>MALLTPIPSPMVNLTQVIDPTEQLAYFPKITFERLKNYDTSSNYAKGKLTRNYMILLPWQHVNRYNFVFSSTGCKVSLKTCIGKLMKDLNPKVLYFIGEGAGNWMARTACEYPDIKFVYRSLKDDLDHHYPLEYQRVIGELSRIIDSGEGLSMETTDATQKTHWDLIHRVSKDALLITLCDAEFKDRDDFFKMVILWRKHVLSCRICTTYGTDLYLFAKYHAKDCNVKLPFFVRSVATFIMQGSKLSGSECYILLTLGHHNNLPCHGEIQNSKMKIAVCNDFYAAKKLDNKSIEANCKSLLSGLRIPINKKELNRQRRLLTLQSNHSSVATVGGSKVIESKWLTNKA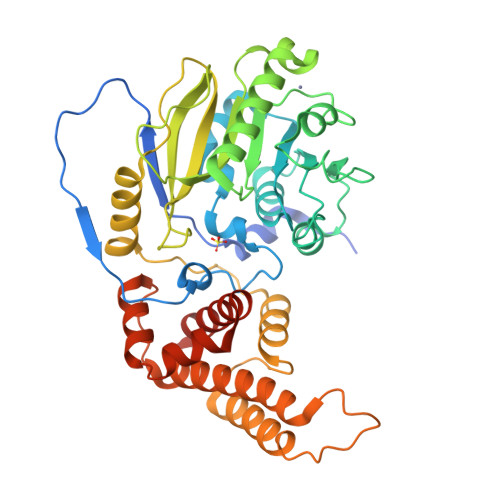NTIIDWLEHILNSPKGELNYDFFEALENTYPNMIKLIDNLGNAEIKKLIKVTGYMLVSKKSGHHHHHH[2x]> MDFSRNLYDIGEQLDSEDLASLKFLSLDYIPQRKQEPIKDALMLFQRLQEKRMLEESNLSFLKELLFRINRLDLLITYLNTRKEEMERELQTPGRAQISAYRVMLYQISEEVSRSELRSFKGGLQEEISKCKLDDDMNLLDIFIEMEKRVILGEGKLDILKRVCAQINKSLLKIINDYEEFSKERSSSLEGSPDEFSNGEELCGVMTISDSPREQDSESQTLDKVYQMKSKPRGYCLIINNHNFAKAREKVPKLHSIRDRNGTHLDAGALTTTFEELHFEIKPHDDCTVEQIYE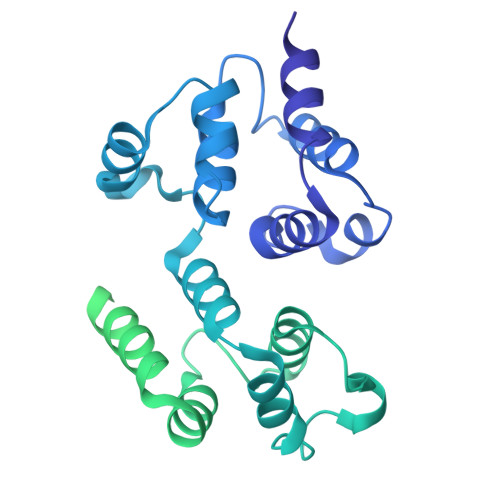ILKIYQLMDHSNMDCFICCILSHGDKGIIYGTDGQEAPIYELTSQFTGLKCPSLAGKPKVFFIQAAQGDNYQKGIPVETASEEQPYLEMALSSPQTRYIPDEADFLLGMATVNNCVSYRNPAEGTWYIQSLCQSLRERCPRGDDILTILTEVNYEVSNKDDKKNMGKQMPQPTFTLRKKLVFPSD> GGPIESAKIFKEFLEDYESGKKSFREASYDA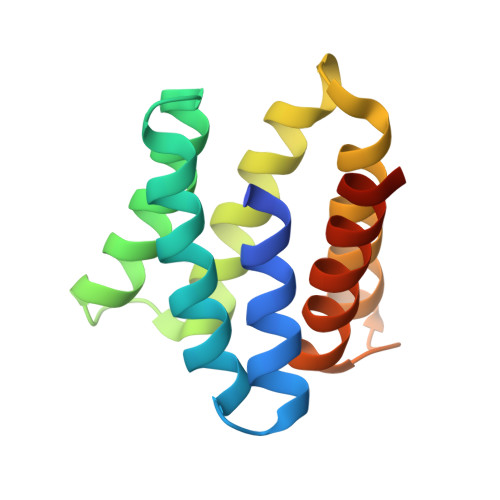TVKLFLWFLPRNIELAEIALRWLIMLESKKVSFEEASLIALREALRWFKVRNNELYKIIKEALDDYESGKKSFEEALWDYYEKVLEYLLKSGGSG> MKIDLNADLGEGCASDAELLTLVSSANIACGFHAG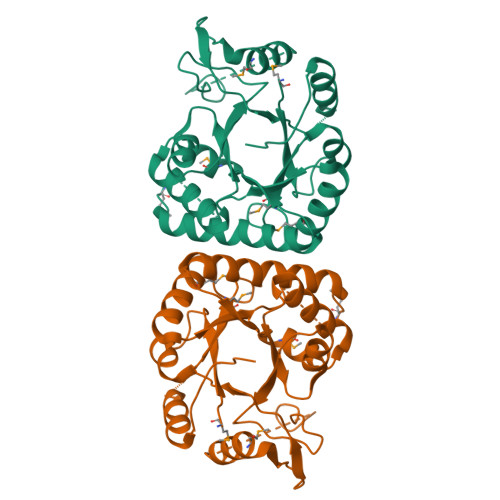DAQIMQACVREAIKNGVAIGAHPSFPDRENFGRSAMQLPPETVYAQTLYQIGALATIARAQGGVMRHVKPHGMLYNQAAKEAQLADAIARAVYACDPALILVGLAGSELIRAGKQYGLTTREEVFADRGYQADGSLVPRSQSGALIENEEQALAQTLEMVQHGRVKSITGEWATVAAQTVCLHGDGEHALAFARRLRSAFAEKGIVVAALEHHHHHH> RGSHMPSPMEDIEEILITEEQLKAKVKELGEMITRDYEGKDLVLIGVLKGAIMFMSGLSRAIDLPLSIDFLAVSSYGSSTKSSGIVKIIKDHDIDIEGKDVLIVEDIIDSGLTLAYLRETLLGR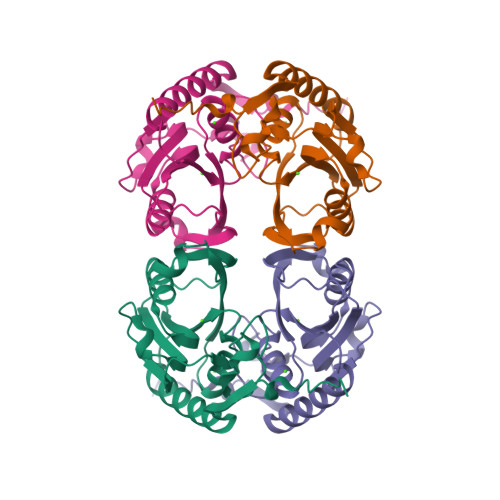KPRSLKICTILDKPERREADVKVDYCGFKIPDKFVVGYGIDYAEKYRNLPFIGVLKPELYK>MAADIFAKFKKSMEVKFTQEYGSNKQAGGDITGKTEKFLRLGPEQDARKQEMIKAGKEIAEKRGIAFYNPMMHMGAPLGQRAITPYTISGTDIVAEPDDLHYVNNAAMQQMWDDIRRTCIVGLDMAHETLEKRLGKEVTPETINHYLETLNHAMPGAAVVQEMMVETHPALVDDCYVKIFTGDDELADEIDKQYVINVNKMFSEEQAAQIKASIGKTTWQAIHIPTIVSRTTDGAQTSRWAAMQIGMSFISAYAMCAGEAAVADLSFAAKHAALVSMGEMLPARRARGPNEPGGLSFGHLSDIVQTSRVSKDPAKIALEVVGAGCMLYDQIWLGSYMSGGVGFTQYATAAYTDDILDNNTYYDVDYINDKYNGAANLGTDNKVKATLDVVKDIATESTLYGIETYEKFPTALEDHFGGSQRATVLAAASGVACALATGNANAGLSGWYLSMYVHKEAWGRLGFFGFDLQDQCGATNVLSYQGDEGLPDELRGPNYPNYAMNVGHQGGYAGIAQAAHSGRGDAFTVNPLLKVCFADELMPFNFAEPRREFGRGAIREFMPAGERSLVIPAK[2x];>[2x]MSDTVDIYDDRGKLLESNVDIMSLAPTRNAAIKKIILDTKRSVAVSLAGIQGALASGKMGGKGRQILGRGLNYDLVGNADAIAENVKNLVQVDEGDDTSVKVIKGGKSLLIQAPSSRIAAGADYMSATTVGAAAVTQTIIDMFGTDMYDAPIAKSAVWGSYPQTMDLMGGNVQGVLSIPQNNEGLGFSLRNIMANHIAAITSRGAMNAAALSSIYEQSGIFEMGGAVGMFERHQLLGLACQGLNANNVVYDIVKENGKDGTIGTVIESIVGRAVEDGVISVDKTAPSGYKFYKANDVPMWNAYAAAGTLAATFVNCGAGRAAQNVSSTLLYFNDILEKETGLPGCDYGKVQGVAVGFSFFSHSIYGGGGPGVFNGNHVVTRHSRGFAIPCVCAAVALDAGTQMFTIESTSGLIGDVFGSIEEFRQPIKAVAGAL;>MAYEAQYYPGATSVGANRRKHMSGKLEKLREISDEDLTAVLGHRAPGSDYPSTHPPLAEMGEPACSIREAVAATPGAAAGDRVRYVQFADSMYNAPATPYFRSYFAAINFRGVDPGTLSGRQIVEARERDMEQCAKVQMETEMTDPALAGMRGATVHGHSVRLQEDGVMFDMLDRRRLEGGVIIMDKDQVAIPLDR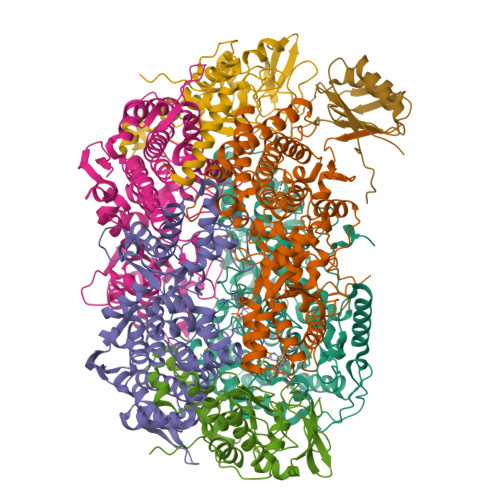KVNLGKPMSSEEAAKRTTIYRVDNVAFRDDAEVIEWVHRVFDQRTSYGFQPK[2x];> MDYKDDDDKGGGWSHPQFEKGGGMSDSASNTEDSIQIEIFPSRILSPETAQKLISELYQVDGIIRVMVQGPRLPERVSAGPGTGEKVEHPLRKPIQIGDQVIELKISVGRIRLEIENAETKEKVRSVCDKMLPFSFEFREGHFLRRKPTVTDYAKLGPETDPRLLGMVDPKAKVNQLVFIEKREKEDDTDKDE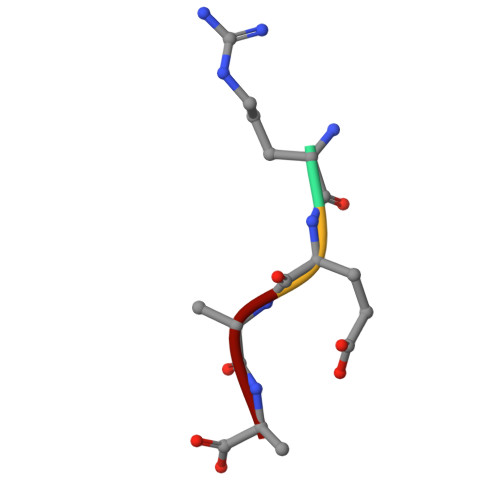> REAA>[4x]METALYLLPVTLGDTPLEQVLPSYNTEIIRGIRHFIVEDVRSARRFLKKVDREID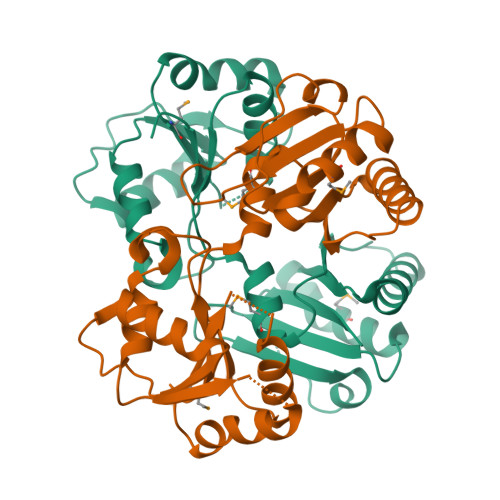IDSLTFYPLNKHTSPEDISGYLKPLAGGASMGVISEAGCPAVADPGADVVAIAQRQKLKVIPLVGPSSIILSVMASGFNGQSFAFHGYLPIEPGERAKKLKTLEQRVYAESQTQLFIETPYRNHKMIEDILQNCRPQTKLCIAANITCEGEFIQTRTVKDWKGHIPELSKIPCIFLLYKLEHHHHHH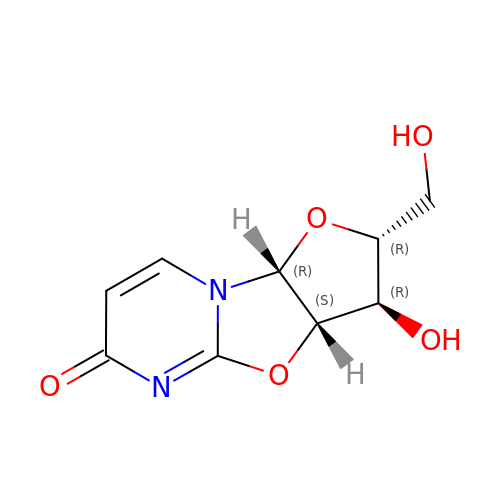2,2'-Anhydro-(1-beta-D-arabinofuranosyl)uracil | C9 H10 N2 O5 | UUGITDASWNOAGG-CCXZUQQUSA-N MLLs degrade N-acyl-L-homoserine lactones (AHLs), molecules that are used in a microbial communication system called quorum sensing (QS) to coordinate a variety of behaviors, including virulence and biofilm formation. We provide the structural and biochemical analysis of the lactonase GcL (WP_017434252.1), isolated from the thermophilic bacteria Parageobacillus caldoxylosilyticus. GcL is a thermostable, highly proficient lactonase with broad substrate specificity (kcat/KM values range between 104 to 106 M–1 s–1) for substrates such as N-butyryl (C4) L-homoserine lactone (HSL) and N-decanoyl (C10)-HSL. The binuclear center, common to all MLLs, is coordinated by five histidine residues and two aspartic acid residues.

We report here the kinetic characterization of several variants, including Ala157Gly, Ala157Ser, Gly156Pro and Ile237Met. The Gly156Pro variant exhibits larger changes in preference, with a 254-fold drop in catalytic efficiency against C6-HSL. Intriguingly, the decrease in substrate preference does not change linearly with the increase in chain length but shifts 2.3 and 6.8-fold for C8- and C10-HSL, respectively. This suggests that subtle substrate conformational sampling may occur differentially as a function of chain length (and, by extension, as a function of the acyl chain hydrophobic character and entropy). To gain some molecular insights into the effects of these substitutions on the active site configuration, structures were solved for both Gly156Pro and Ile237Met variants. The structure of the Gly156Pro variant reveals that the Asn152-Ala157 loop is significant in accommodating long chain AHL substrates. The conformational change in this loop may be responsible for the altered substrate preference of the enzyme. We used MDpocket70 to locate the hydrophobic/hydrophilic regions of the cavity along with the MD simulations of C6-, and C8-HSL in complex with wild-type GcL and Gly156Pro variant. Interestingly, the end of the C6-HSL acyl chain, which is the most mobile part of the substrate, lays in the same position as the rearranged residue Glu155 side chain, creating strong repulsion and destabilizing the substrate. In contrast, the end of the C8-HSL acyl chain lies further from the active site and the repulsion between Glu155 and the substrate tail is diminished, allowing tighter binding of C8- compared to C6-HSL.

>[3x]WSHPQFEKENLYFQSMANVIKARPKLYVMDNGRMRMDKNWMIAMHNPATIHNPNAQTEFVEFPIYTVLIDHPEGKILFDTSCNPNSMGPQGRWAESTQQMFPWTATEECYLHNRLEQLKVRPEDIRYVVASHLHLDHAGCLEMFTNATIIVHEDEFNGALQCYARNQKEPAYIWADIDAWIKNNLQWRTVKRHEDNILLAEGVKVLNFGSGHAWGMLGLHVELPETGGIILASDAIYTAESYGPPIKPPGIIYDSLGYMNTVERIRRIAQETKSQVWFGHDAEQFKKFRKSTEGYYE>[6x]DAPAMKDKSKSHEEEKTDPTAGAHAPVVFTLRTGIAEGRMVYIGVGGDIDHKINPTLVVHE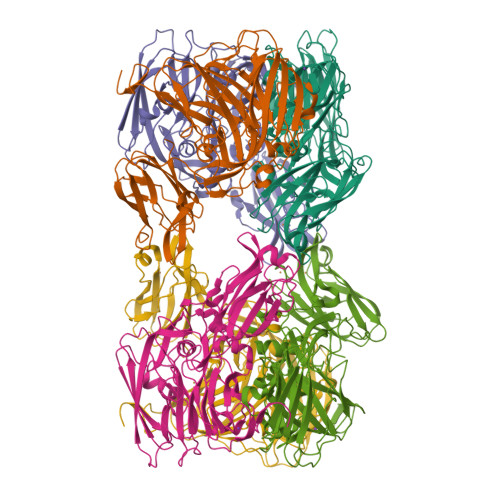GETVQVNLVNGEGAQHDVVVDQYAARSAIVNGKNASSTFSFVASKVGEFNYYCSIAGHRQAGMEGNIQVLPGNRAEMKSSGADITRDPADLPGPIGPRQAKTVRIDLETVEVKGQLDDNTTYTYWTFNGKVPGPFLRVRVGDTVELHLKNHKDSLMVHSVDFHGATGPGGAAAFTQTDPGEETVVTFKALIPGIYVYHCATPSVPTHITNGMYGLLLVEPEGGLPQVDREFYVMQGEIYTVKSFGTSGEQEMDYEKLINEKPEYFLFNGSVGSLTRSHPLYASVGETVRIFFGVGGPNFTSSFHVIGEIFDHVYSLGSVVSPPLIGVQTVSVPPGGATIVDFKIDRAGRYILVDHALSRLEHGLVGFLNVDGPKNDSIMHEGPAKQ>TEQATTTDELAFTRPYGEQEKQILTAEAVEFLTELVTHFTPQRNKLLAARIQQQQDIDNGTLPDFISETASIRDADWKIRGIPADLEDRRVEITGPVERKMVINALNANVKVFMADFEDSLAPDWNKVIDGQINLRDAVNGTISYTNEAGKIYQLKPNPAVLICRVRGLHLPEKHVTWRGEAIPGSLFDFALYFFHNYQALLAKGSGPYFYLPKTQSWQEAAWWSEVFSYAEDRFNLPRGTIKATLLIETLPAVFQMDEILHALRDHIVGLNCGRWDYIFSYIKTLKNYPDRVLPDRQAVTMDKPFLNAYSRLLIKTCHKRGAFAMGGMAAFIPSKDEEHNNQVLNKVKADKSLEANNGHDGTWIAHPGLADTAMAVFNDILGSRKNQLEVMREQDAPITADQLLAPCDG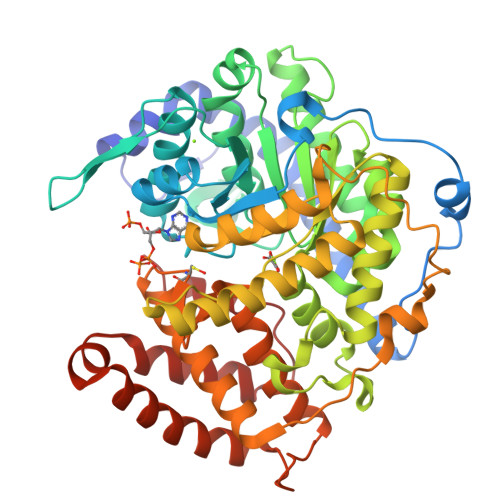ERTEEGMRANIRVAVQYIEAWISGNGCVPIYGLMEDAATAEISRTSIWQWIHHQKTLSNGKPVTKALFRQMLGEEMKVIASELGEERFSQGRFDDAARLMEQITTSDELIDFLTLPGYRLLA[2x]> MAHHHHHHMLNNNQNNKKMSSSSKLRLLSDLQQLQKDPPEGITASPESENDLYVWNATITGPMDSIWEGGIFFLRLTFPEDYPTKPPKVKFTSKIFHPNVYKDGSICLDIVQDKWSPIYTVDSILTSILSLLEDPNP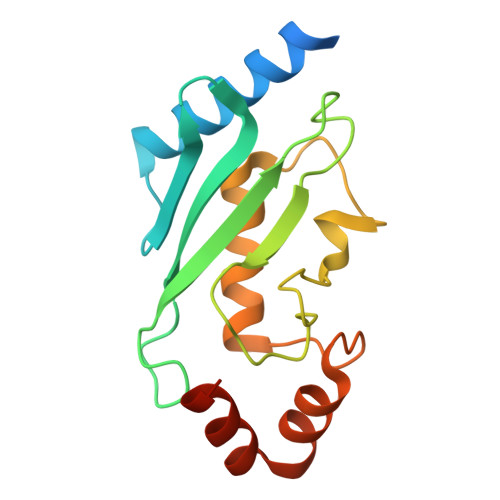DSPANPEAAKLFVNDPKEYKKRVRKCVESLME>[6x]EAGGVFKLIANDGKADRMIMANDLLNDRIKSIMCLRAKQGFSDPTPTLVDIERTHILLINSHYKPFAAMGYEYQKTRPNTGNPTYNSTIQFSIPQFGDFFSDMVVHVQLAATSASAGTVPALPAFIGADDQVLTSTSVVSATENTTSGVYTLYTQSYVNQQGTTQTVAAAATNFVRYCEYPGLRLFKRVKFEVNGNPLDEYTALAAIMYNKFHVPDFKLTGWKRLIGQEVPVEAASNLVNIASTTPWGSPIVALSDVNGTAVTGSPV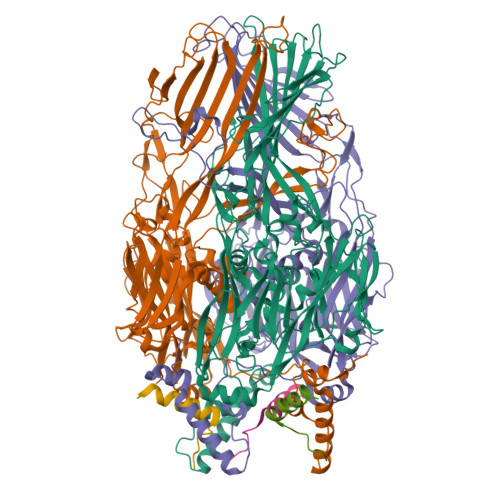NAAITARKLTQVVFGAQTPKATQEQLNMFVPLLFWFRDPRLAIASVSIPYGQRFITVDIEQQSNILFTAPGNLFLQTTVETLLTTGAGKGTATGVLLTQYNRYTTYTPTLASGSSIDGTQAVQNIELYINNIFVTPEIHDIYIKRIGFTLIRVYREQVQREVNAADQVLQSQLKWPVEFIYLGLRPANNIAAGNTYQWRDWHHLTSVTNEPVYDVSQSYARVSIDDTVAPVGSTTFKQSASQVMQNQYIVPVETETLDTVRVKAHGIELYAQYRAQFYRDYIPWNYGSFNLVTPQDKGALFLNFCLYPGTYQPSGHVNISRAREFYIEYTSSFCDSSNPCDLISIAKCINFLLISDGSAVLRYSTKEFYLQCLILRCI>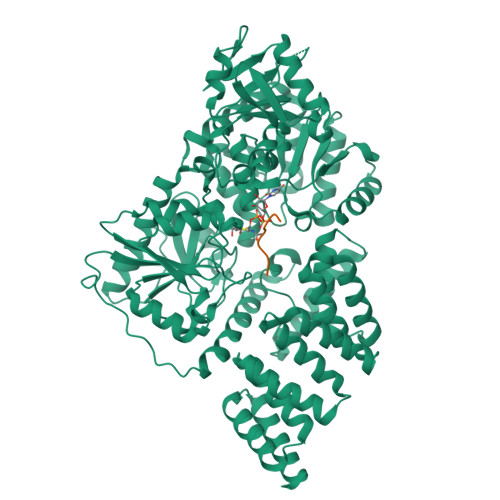[4x]GPGSCPTHADSLNNLANIKREQGNIEEAVRLYRKALEVFPEFAAAHSNLASVLQQQGKLQEALMHYKEAIRISPTFADAYSNMGNTLKEMQDVQGALQCYTRAIQINPAFADAHSNLASIHKDSGNIPEAIASYRTALKLKPDFPDAYCNLAHCLQIVCDWTDYDERMKKLVSIVADQLEKNRLPSVHPHHSMLYPLSHGFRKAIAERHGNLCLDKINVLHKPPYEHPKDLKLSDGRLRVGYVSSDFGNHPTSHLMQSIPGMHNPDKFEVFCYALSPDDGTNFRVKVMAEANHFIDLSQIPCNGKAADRIHQDGIHILVNMNGYTKGARNELFALRPAPIQAMWLGYPGTSGALFMDYIITDQETSPAEVAEQYSEKLAYMPHTFFIGDHANMFPHLKKKAVIDFKSNGHIYDNRIVLNGIDLKAFLDSLPDVKIVKMKCPDGGDNADSSNTALNMPVIPMNTIAEAVIEMINRGQIQITINGFSISNGLATTQINNKAATGEEVPRTIIVTTRSQYGLPEDAIVYCNFNQLYKIDPSTLQMWANILKRVPNSVLWLLRFPAVGEPNIQQYAQNMGLPQNRIIFSPVAPKEEHVRRGQLADVCLDTPLCNGHTTGMDVLWAGTPMVTMPGETLASRVAASQLTCLGCLELIAKNRQEYEDIAVKLGTDLEYLKKVRGKVWKQRISSPLFNTKQYTMELERLYLQMWEHYAAGNKPDHMIKPVE;>VTPVSTAA[4x]Lipins are magnesium-dependent phosphatidic acid phosphatases (PAPs) that catalyze the dephosphorylation of the membrane lipid phosphatidic acid (PA) to produce diacylglycerol (DAG). Our principal findings are that the M-Lip domain is a new protein fold that forms a dimer, binds membranes, and can affect lipin PAP activity, oligomerization, subcellular localization, and adipogenesis. Phospholipid synthesis and fat storage as triglycerides are regulated by lipin phosphatidic acid phosphatases (PAPs), whose enzymatic PAP function requires association with cellular membranes.

We, therefore, truncated the M-Lip domain of mouse lipin 1 to remove the C-terminal cluster of hydrophobic and basic residues implicated in membrane binding by HDX-MS. We refer to this construct as the M-Lipxtal domain. The structure of the M-Lipxtal domain of mouse lipin 1 was determined to resolutions of 1.5 Å and 1.9 Å in two unique space groups. Phases were obtained using single-wavelength anomalous diffraction from selenomethionine (SeMet)-derivatized protein. The M-Lip domain of mouse lipin 1 and lipin 2 formed a symmetric or near symmetric dimer in all three crystal forms with a root mean square deviation for all atoms ranging between 0.36–0.77 Å. The observation of near identical dimers in three different crystal structures strongly suggested the native quaternary structure of the M-Lip domain as dimeric. Analysis of the dimer interface of the M-Lip revealed an extensive network of interactions between the two subunits with residues within the α3 helix, which was located in the center of the dimer, mediating the majority of these interactions. SEC-MALS reported a MW of 25.6 ± 0.6 kDa for the mouse lipin 1 M-Lipxtal domain, which was consistent with the MW of 26 kDa for a M-Lipxtal dimer.

>[2x]SLRDLPSIAISLCGGLSDHREITKDAFLEQAVSYQQFADNPAIIDDPNLVVKVGNKYYNWTTAAPLLLAMQAFQKPLPKATVESIMRDKMP>[2x]CUGGGCGG;>CCGCCUGG[2x]

We have obtained crystals of a racemic compound consisting of l- and d-RNA duplexes in which the enantiomers pack in the crystal lattice in an asymmetric manner and show differences in their structures, crystal contacts and interactions with the solvent. The crystals of d- and l-RNA duplexes (CUGGGCGG)-(CCGCCUGG) belong to space group P1 with the unit cell parameters a = 21.1 Å, b = 26.7 Å, c = 39.1 Å, α = 105.9°, β = 97.0°, and γ = 91.6°. The unit cell contains one d-RNA duplex and one l-RNA duplex stacking head-to-tail, arranged in the crystal lattice into parallel semi-infinite columns. The d-duplexes have the helical parameters characteristic of A-RNA, while the l-duplexes take values appropriately inverted for the other enantiomer.

The absolute configuration of the structure was determined for each analyzed crystal using the anomalous dispersion of X-rays from the Zn2+ ions. Of the nine crystals that gave diffraction data containing statistically significant anomalous signals, seven crystals had the K:L RNA duplex in the d-configuration, and the M:N duplex was in the l-configuration. The remaining two crystals had the inverted configuration l-(K:L)/d-(M:N). Of the eight crystals that gave no statistically significant anomalous signal but gave anomalous peaks at the Zn2+ ions, four crystals were d-(K:L)/l-(M:N), and four were l-(K:L)/d-(M:N). The ratio of the d-(K:L)/l-(M:N) to l-(K:L)/d-(M:N) crystal structures, of 7 to 2 for the best data sets and 11 to 6 overall, does not indicate a clear bias. The intermolecular crystal contacts of the two enantiomers are also different. When the two duplexes (K:L and M:N) are compared, chain K is more exposed to the solvent than its corresponding enantiomer, chain M, which makes more extensive contacts with neighboring RNA molecules. The percentage ratio of the solvent-exposed surface area to the intermolecular crystal contact area is 72/28 for chain K and 57/43 for chain M. The situation is reversed for the other strands of the two duplexes: the ratios of the solvent-exposed intermolecular contact areas are 55/45 for chain L and 71/29 for chain N. Asymmetry between the RNA enantiomers is also observed in their interactions with the Zn2+ ions. In the presented structure, one enantiomer interacts with three zinc cations, while the other interacts with four zinc cations.> APLAQQTCANNRHQCSVHAECRDYATGFCCRCVANYTGNGRQCVAEGSPQRVNGKVKGRIFVGSSQVPVVFENTDLHSYVVMNHGRSYTAISTIPETVGYSLLPLAPIGGIIGWMFAVEQDGFKNGFSITGGEFTRQAEVTFLGHPGKLVLKQQFSGIDEHGHLTISTELEGRVPQIPYGASVHIEPYTELYHYSSSVITSSSTREYTVMEPDQDGAAPSHTHIYQWRQTITFQECAHDDARPALPSTQQLSVDSVFVLYNKEERILRYALSNSIGPVRDGSPDA;> APLAAPSKPIMVTVEEQRSQSVRPGADVTFICTAKSKSPAYTLVWTRLHNGKLPSRAMDFNGILTIRNVQPS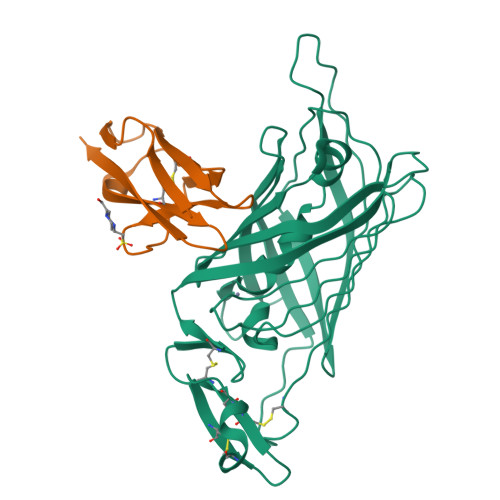DAGTYVCTGSNMFAMDQGTATLHVQV>SLQKQEYKTLEYNLTTTEVVMENVTAFWEEGGTPVLKDINFKIERGQLLAVAGSTGAGKTSLLMMIMGELEPSEGKIKHSGRISFCSQFSWIMPGTIKENIIFGVSYDEYRYRSVIKACQLEEDISKFAEKDNIVLGEGGITLSGGQRARISLARAVYKDADLYLLDSPFGYLDVLTEKEIFESCVCKLMAN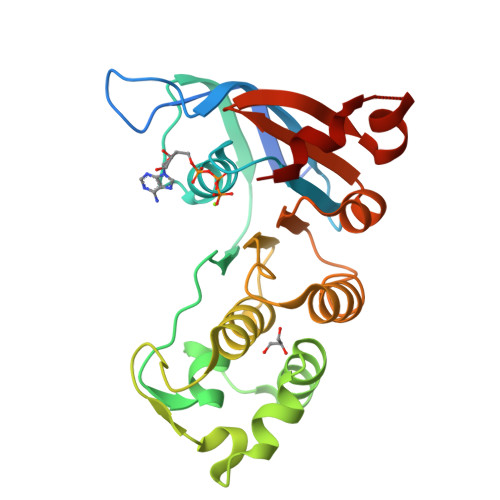KTRILVTSKMEHLKKADKILILHEGSSYFYGTFSELQNLQPDFSSKLMG[2x]XYLULOSE-1,5-BISPHOSPHATE 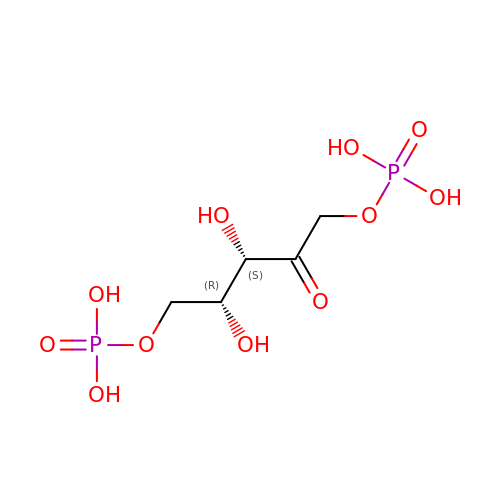| C5 H12 O11 P2 | YAHZABJORDUQGO-WUJLRWPWSA-N> MARVTTGITSSHIPALGAAIQTGTSDNDYWGPVFKGYQPIRDWIKQPGNMPDVVILVYNDHASAFDMNIIPTFAIGCAETFKPADEGWGPRPVPDVKGHPDLAWHIAQSLILDEFDMTIMNQMDVDHGCTVPLSMIFGEPEEWPCKVIPFPVNVVTYPPPSGKRCFALGDSIRAAVESFPEDLNVHVWGTGGMSHQLQGPRAGLINKEFDLNFIDKLISDPEELSKMPHIQYLRESGSEGVELVMWLIMRGALPEKVR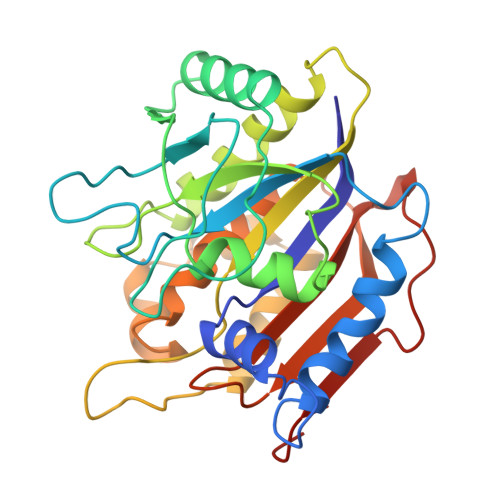DLYTFYHIPASNTALGAMILQPEETAGTPLEPRKVMSGHSLAQA>[2x]MKKLFLVFWWHMHQPLYREPYTGEYLLPWTFFHAVKDYYDMPAYLKDFEIKLNFNLTPVLIDQIQEYAQGKAKDVFLEAIRKDPDDLEKEEVEKLIEFTKLNYEKPIYRFERIRELMNKEKLNREELLDLQTLNLLAWCGRTLRKDLKDLLNKGRNYTQEEKEYVLNKYFEIIKKTLSIYREIKEEGKGSVSTSPYYHPLIPILLNPNCVYETTPNVKIPD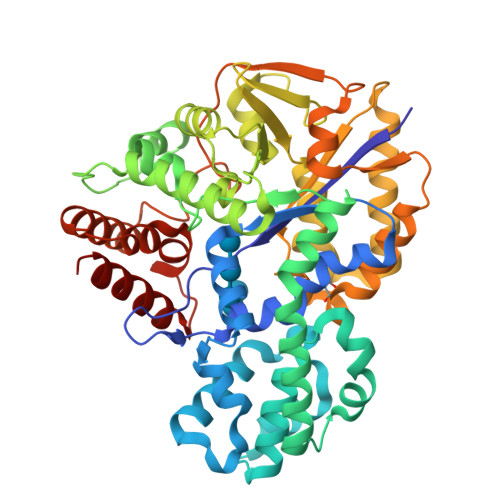FAVSFREDASKHVELAKEKYFEIFGEHPVYMWPPEASVSNEALELYYEKGINMLATDEVILKNSVERASPYLRYYFRELISVFFRDKTLSDLIGFSYHAWNAEDAVRDFIGRLKKIHESVDFQPVVFVVLNGENCWEYYEENGIPFLEKLYSTLEKEEWIETLTLEEAMRKEDVKTEVIESVKAGTWFDGNFLKWIGNKEKNEYWKILIEAKKKAKNDYILVAEGSDWFWWQGEEKAPFVEVFDKLFRSFVRRAQE>IDPNAQLTTAQLQTYGDLSMMEIYRNYHYAFTQQLMGCWNTTNYGGRHTLDNNEMSRIWTSFYTQSLKNIIDAQYRTAEDAEKVNINSVLRIYRVYLMSIITDTYGDAPFSEAGLGFLEGKFNPKYDKQEDIYNAFFLELEDAVNKIDPTKDKVTGDLIYAGDVTKWQQLANSLRLRFAMRISSVNPTKAQTEFENALAANGGVITDASSDALIKYMTIAFSFGQEAYSDYRGNSLSQLLFGNDPANNPSYLCSTFFNQLYNSGDPRTFKISRCYYDGLMSATSPDNRVDITQEMIEKGIAFSPRDPGAYSWEPWPTGYDSDICAELAVNNPSVTATMAREVEPKLANNFLKSDNPGVVMTSAEVKFLMAEATVKKWNVGSVSAEDLYKQGVRAAIDFLTDNYGCTATTDAEFDAFIQDKGAFGHTDNQKLEAINTQAWILHFTNPAECWANVRRSGYPKLKSPAEYGFGQYLTGG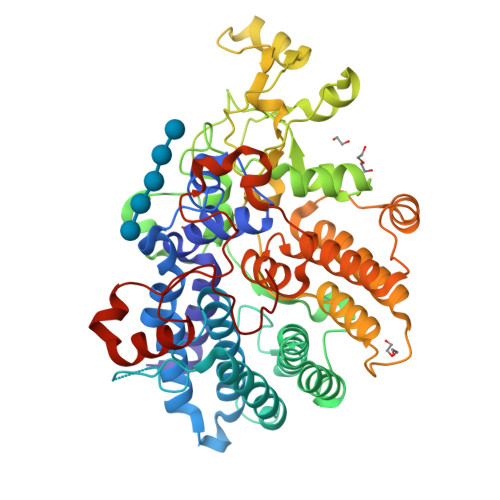TEIPVRLCYPVLESSYNKKSYNEAIERMGGTDNWHSLLWWDTEN[10x]> MGSDKIHHHHHHENLYFQGMKIKVALLDKDKEYLDRLTGVFNTKYADKLEVYSFTDEKNAIESVKEYRIDVLIAEEDFNIDKSEFKRNCGLAYFTGTPGIELIKDEIAICKYQRVDVIFKQILGVYSDMAANVATISGENDKSSVVIFTSPCGGVGTSTVAAACAIAHANMGKKVFYLNIEQCGTTDVFFQAEGNATMSDVIYSLKSRKANLLLKLESCIKQSQEGVSYFSSTKVALDILEISYADIDTLIGNIQGMDNYDEIIVDLPFSLEIEKLKLLSKAWRIIVVNDGSQLSNYKFMRAYESVVLLE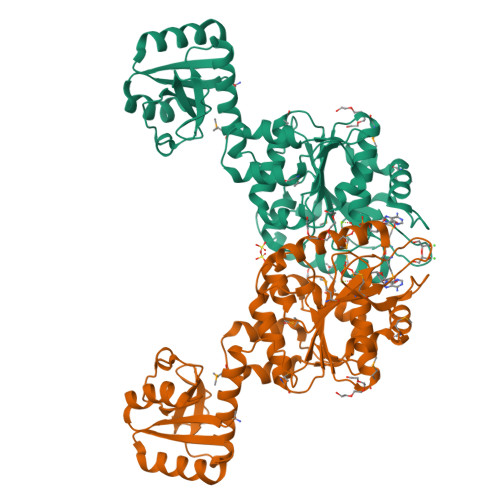QNDDINIIRNMNMIYNKFSNKNSEMLSNISIKTIGGAPRYEHATVRQIIEALTKMEFFEEILQ>PPGPPGPRGPPGPPGPPGGPGPPGPPGX[3x]

Collagen's structure involves the assembly of three polyproline II helices, with each individual chain consisting of a three residue repeat sequence with the general form (Glycine–Xaa–Yaa). Within collagen's trademark triple-helical structure, three polyproline II helices are stitched together by a network of interstrand hydrogen bonding along the central axis of the right-handed triple helix. The triple helix is stabilized by the backbone NH groups of the Gly residues acting as hydrogen bond donors to the carbonyl oxygen of Xaa position residues in neighboring chains. To gain atomic level insight into these new rules we present two high-resolution crystal structures of collagen triple helices, with the first peptoid-containing collagen peptide structure.

We solved the structure of the CMP 25, bearing the Xaa position NmetG residue, with the sequence [H–(POG)2(PRG)(POG)3(NmetG–OG)(POG)2–NH2] to 1.15 Å resolution. In addition, we have reported two new collagen crystal structures, with the first structure of a collagen triple helix containing a peptoid residue. In the NmetG structure, the void in space observed along the surface of the triple helix in the Val structure is filled by the N-methyl group of NmetG. This prevents the NH backbone–water interaction from occurring and better protects the Gly Cα from solvent exposure, with the nearest water being positioned approximately 3.7 Å away from the backbone NH and approximately 3.5 Å away from the Gly Cα. If there is any other residue present in the Xaa position, this average drops to 3.4 ± 0.2 Å. These observations are consistent with our structures, with the NmetG residue blocking solvent to a greater extent than the Val residue. Beyond solvent exposure, the identity of the Xaa position residue will affect the backbone dihedral angles of nearby residues. Averaging φ angles of Gly residues from collagen structures in the PDB gives a value of −69 ± 5° while averaging ψ angles gives a value of −176 ± 5° or 173 ± 5°.32 In our structure, the Gly residues adjacent to the Xaa NmetG residue adopt conformations closely matching the PDB average Gly (φ, ψ) angles with average values of (−68°, 176°) (Fig. 5d and Table S4†). Comparing these angles to other structures in the PDB, the Gly residues next to NmetG adopt conformations similar to those adopted by Gly residues adjacent to either Pro or Hyp residues.>[8x]MDVGKLESFIVEKMAERKVPGISISIIKDGD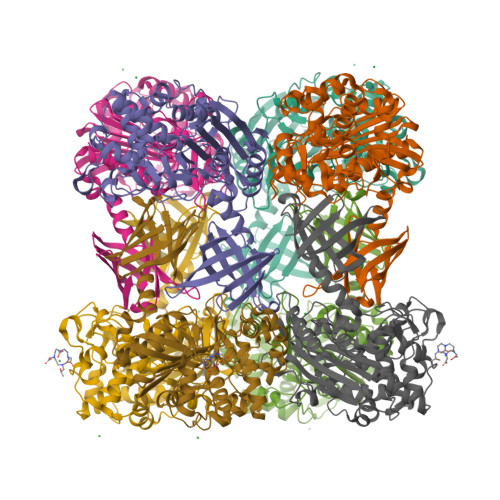VVYAKGFGYRNVEARLPSTPETIYGIGSITKSFTALAIMKLVEEGGLSLDDPVEKFVNIKLRPFGEPVTVHHLLTHSSGIPSLGYAEAFIDGMVGGDNWLPVSTPEETIAFARDMEKWAVAKPGERFFYLNTGYVLLGKIIEKVSGVSYEEYIKKKILEPLGMNRSYFFKEEVEKDKDVAMGYILDKEGRLVPQPFPYGITADGGLLSSVLDLAKYLKMYIERDESIVSKEYIEKMETSYIKVPWEIFGGEGYGYGLIIYPNFLGEKLVGHSGSVGMYTGYIGYIPEKKIGVAVLENSSGYPPSYIAMYALALLLGKNPEKELPFIYRERILKKVEGRYMGYKGTIKFEVKVDGDVVYLRALGRAFTYTIPLFPEVLEEDFIKCYTLSNGRKMYAEFYIKDNKVDLIFERYRLIKS>LDRADILYNIRQTSRPDVIPTQRDRPVAVSVSLKFINILEVNEITNEVDVVFWQQTTWSDRTLAWNSSHSPDQVSVPISSLWVPDLAAYNAISKPEVLTPQLARVVSDGEVLYMPSIRQRFSCDVSGVDTESGATCRIKIGSWTHHSREISVDPTTENSDDSEYFSQYSRFEILDVTQKKNSV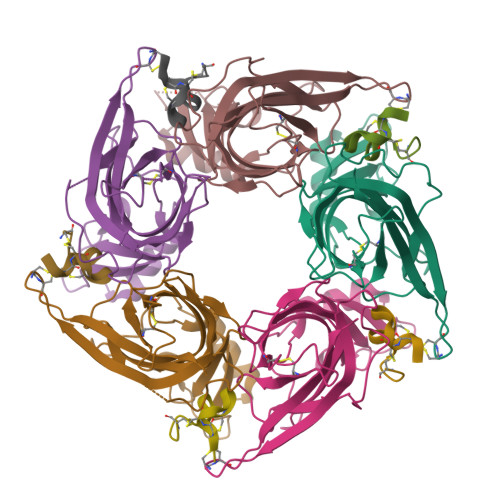TYSCCPEAYEDVEVSLNFRKKGRSEIL[5x];>[5x]SGCCSNPACRVNNPNICX> MQDKIPTIAELRELSLRLLTKIPYLKMLVLFGSRATGNINANSDWDFAVLYDEEKYNLYIQNNPLAAFVIPGILGEIFKINSDKIDIVELNHCSKLI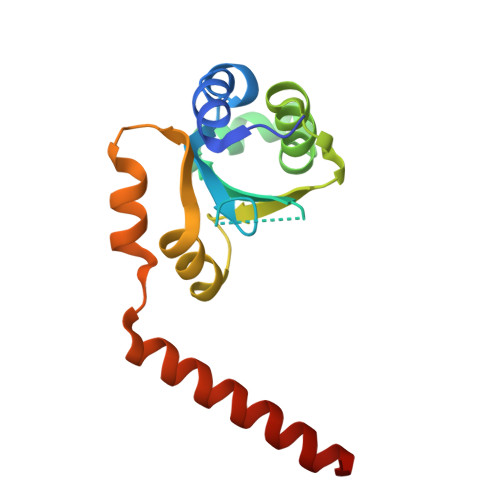AHFVARDGKVLYEEPGDEFDKFQQRVLLSNTEIKKIEKTKLENIENFLQRWGV4-chloranyl-N-[[4-chloranyl-3-(3-chloranyl-5-cyano-phenoxy)-2-fluoranyl-phenyl]methyl]-2-(hydroxymethyl)-1H-imidazole-5-carboxamide 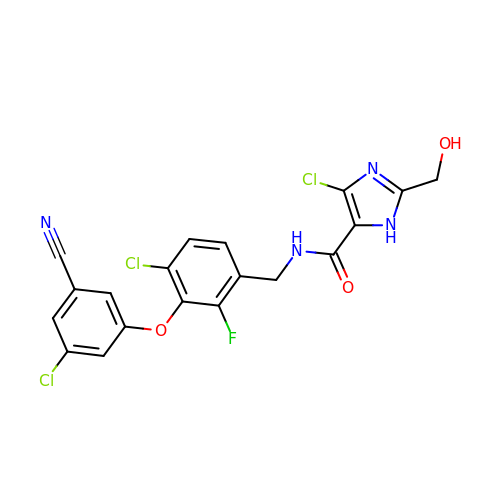| C19 H12 Cl3 F N4 O3 | AASNTQJUPFQRBO-UHFFFAOYSA-N3-(5-AMINO-7-HYDROXY-[1,2,3]TRIAZOLO[4,5-D]PYRIMIDIN-2-YL)-N-(3,5-DICHLOROBENZYL)-BENZAMIDE | C18 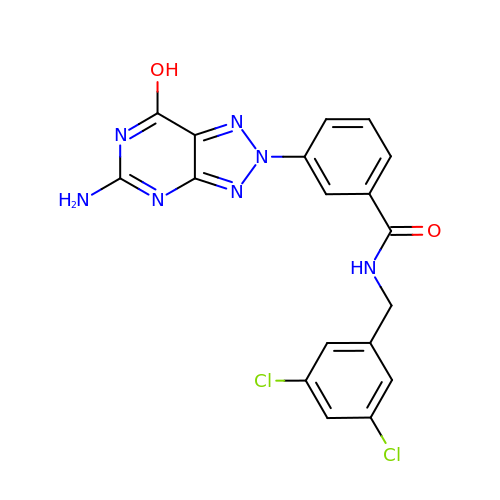H13 Cl2 N7 O2 | JMQTXEWNXSPEKX-UHFFFAOYSA-N To confer the favorable attributes of ABEs upon a CBE, we envisioned transforming TadA into an enzyme capable of robust cytidine deamination and subsequently generated an improved class of CBEs that uses TadA instead of a naturally occurring cytidine deaminase. Here we describe the development of two families of base editors, CABE-Ts and CBE-Ts, which use variants of TadA to catalyze the deamination of cytosines with either retention (CABE-Ts) or loss (CBE-Ts) of adenine deamination. To illuminate how amino acid substitutions identified from directed evolution affect TADAC’s substrate tolerance, we determined crystal structures of TadA*8.20 from ABE8.20-m13, the template used to evolve CABE-T1, and TADAC-1 variants from CABE-T1 reported here. Through X-ray crystallography, we show how the accumulation of substitutions impacts the shape of the active site cavity and may contribute to the accommodation of cytosine as substrate and the subsequent shift in specificity toward C-to-U deamination.

In addition to the perturbations on the right side of the TADAC-1.14 active site cavity, evaluation of the TADAC-1.19 structure reveals that other substitutions (E27G and I49N) from our evolution caused major structural changes on the left side of the active site cavity. These structural changes are likely caused by the E27G substitution, which results in the loss of essential hydrogen bonds between E27 and A48, I49 and G50. Because of these hydrogen bond losses, a conformational change occurred that reoriented residue E25 of TADAC-1.19 to a similar position that was formerly occupied by residue E27 in TadA*8.20. The displacement of E25 shortens the α1-helix, changes the length and conformation of the loop between α1 and β1 (D24 to P29) containing the E27G substitution and unfolds α5- and α6-helices, reshaping the TADAC-T1.19 active site cavity and potentially impacting target nucleobase binding within the active site.

>MSEVEFSHEYWMRHALTLAKRARDERGVPVGAVLVLNNRVIGEGWNRANGLHDPTAHAEIMALRQGGLVMQNYRLYDATLYSTFEPCVMCAGAMIHSRIGRVVFGVRNAKTGAAGSLMDVLHHPGMNHRVEITEGILADECAALLCRFFRMPRRVFNAQKKAQSSTD[8x]> MQKLLSPRTARHARLFRLAGKLADSGSPGVPKSDGERLVWVNSHVRRDKDISLSQEEERIRELMMPLEVGENSFAANGQATHGNLFYFREYPMYPGEYVPAEHNTLSSLRDELRLDLTAQSLKEAWMRVSGGVYFQSVDEYYASVDGLDAEQ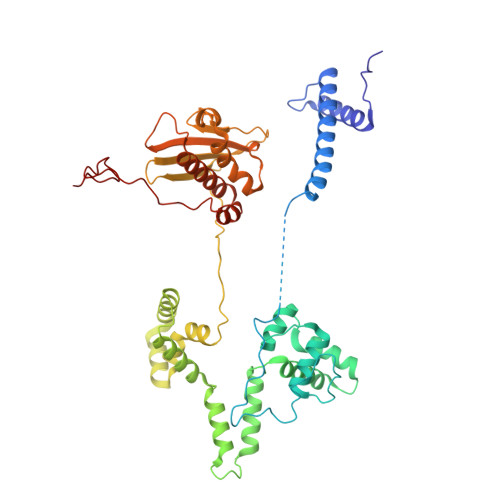IGEVLAALFPELNCYEAQALVQRTLECISRPVSAASRQLSRTITAEAVGLDNAPGHYTNFLEWMGRLTETRAFKTEHALFEFSRRKFNRDDVRVMFENYRLMSKATLLADSADSYSHFYTVLKDFARKVAGEDSRHQIGVRIDEAEVDPETGIAVGRGCADGEKYHFTALLRENRDHNGIITVMGKPLSLVLDNKAWLMEMVLMPFDEANLDYRDFDAHIVSEGHAMPSIANEIAAFALRMAVANALVKLIPLTRIPLKKSGLLSVDRRRERGQFPGYLDGKKVKRRFAKR> MGSSHHHHHHSSGLVPRGHMSLFHLIAPSGYCIKQHAALRGIQRLTDAGHQVNNVEVIARRCERFAGTETERLEDLNSLARLTTPNTIVLAVRGGYGASRLLADIDWQALVARQQHDPLLICGHSDFTAIQCGLLAHGNVITFSGPMLVANFGADELNAFTEHHFWLALRNETFTIEWQGEGPTCRAEGTLWGGNLAMLISLIGTPWMPKIENGILVLEDINEHPFRVERM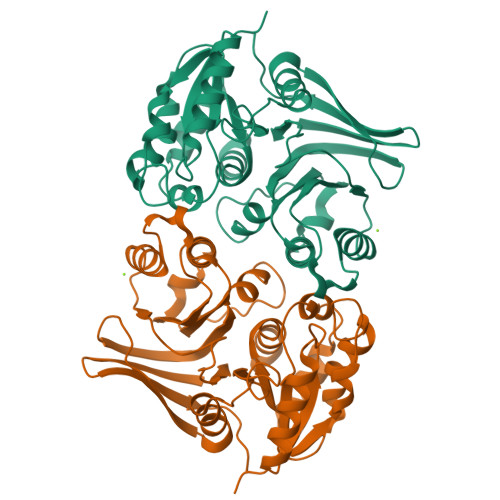LLQLYHAGILPRQKAIILGSFSGSTPNDYDAGYNLESVYAFLRSRLSIPLITGLDFGHEQRTVTLPLGAHAILNNTREGTQLTISGHPVLKM>[3x]MPEGPELHLASQFVNEACRALVFGGCVEKSSVSRNPEVPFESSAYRISASARGK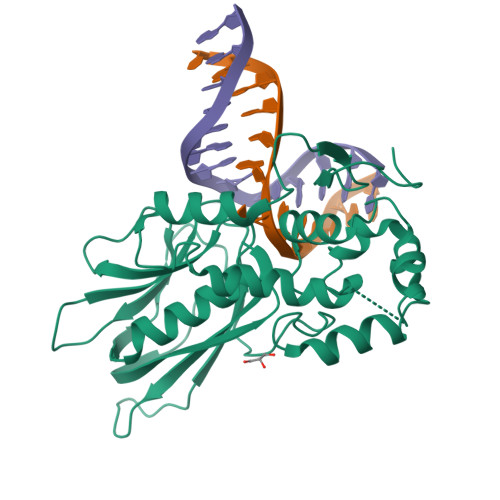ELRLILSPLPGAQPQQEPLALVFRFGMSGSFQLVPREELPRHAHLRFYTAPPGPRLALCFVDIRRFGRWDLGGKWQPGRGPCVLQEYQQFRENVLRNLADKAFDRPICEALLDQRFFNGIGNYLRAEILYRLKIPPFEKARSVLEALQQHRPSPELTLSQKIRTKLQNPDLLELCHSVPKEVVQLGGRGYGSESPEEDFAAFRAWLRCYGMPGMSSLQDRHGRTIWFQGDPGPLAPKGRKS> DKLTQQDYNTDFIYESHHRQPKESLTHASVLSAYTASYKTTAIKSIADNAVVLDIGYGKGNDGPRYAVRPLTVTGIDTAARMLAIADQNKPENVTLVKQGFFTHITKTSNTYTHVIAFNSLHYPLASSHPDTLVQRLPTCPANILIPCHHLLEG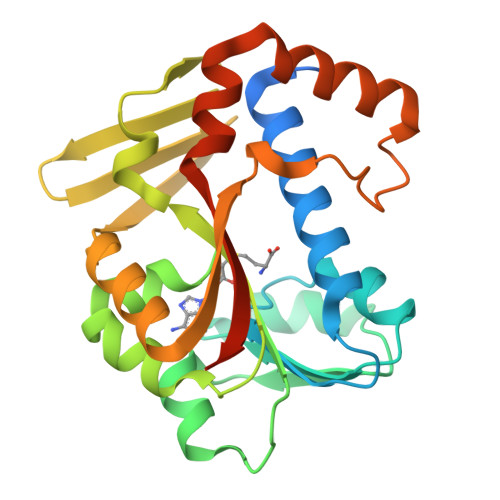IQTPTYSVVKDEDMWCVKVTKNEFIESSYNYDVFVKALESKYHVTIGSLLDCVEKPSTRSITPTLWTAMRNFVNNDQEMQRILSGYITFNLTPLPPKVEIINDWLD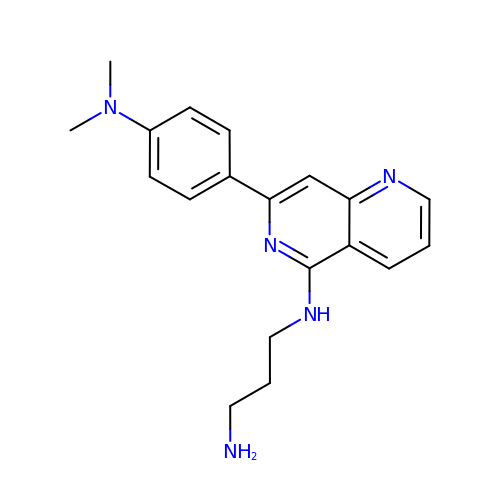N-{7-[4-(dimethylamino)phenyl]-1,6-naphthyridin-5-yl}propane-1,3-diamine | C19 H23 N5 | RIWJHDIYQSQOAT-UHFFFAOYSA-N>[2x]MEFLNSIPWEEVVPGQFTANPGFQVTDYFEIVRQPADGNCFYHSIAELFVPNKNDFSFRLVKQHLELAARRFFEEESEAKGLGLSLEKYLEVAMC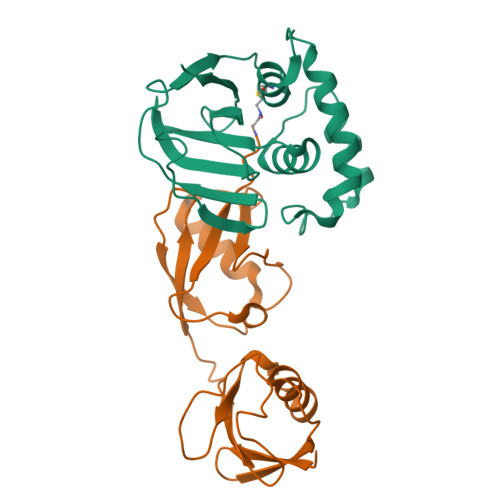DNEWGGSLEASMLAKHLDITIVIWVIEGPSRVAAAVKFGPGDVAGAINLLHTGYNHFDALRLLVDDSQVSRQPRSGSHHHHHH;>[2x]MGGDLKVKMLGGEEILVPLRDSMMVSELKQFIAQKINVPAFQQRLAHLDSREVLQEGVPLVHQGLKAGSTILLMVQNSSATLNILVRNDKGRSSSYEVQLTQTVAVLKQQVCQRERVQADQFWLSFEGKPMDDEHPLGEYGLTTGCTVFMNLRLRG> GAMDITGPIILQTYRAIADYEKTSGSEMALSTGDVVEVVEKSESGWWFCQMKAKRGWIPASFLEPLDSPDETEDPEPNYAGEPYVA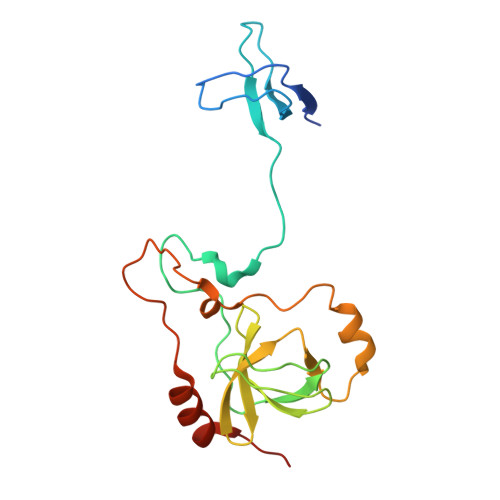IKAYTAVEGDEVSLLEGEAVEVIHKLLDGWWVIRKDDVTGYFPSMYLQKSGQDVSQAQRQIKRGAPPRRSSIRNAHSIHQRSRKRLSQDAYRRNSVRFLQQRRRQAR>LPTSNPAQELEARQLGRTTRDDLINGNSASCADVIFIYARGSTETGNLGTLGPSIASNLESAFGKDGVWIQGVGGAYRATLGDNALPRGTSSAAIREMLGLFQQANTKCPDATLIAGGYSQGAALAAASIEDLDSAIRDKIAGTVLFGYTKNLQNRGRIPNYPADRTKVFCKTGDLVCTGSLIVAAPHLAYGPDARGPAPEFLIEKVRAVRG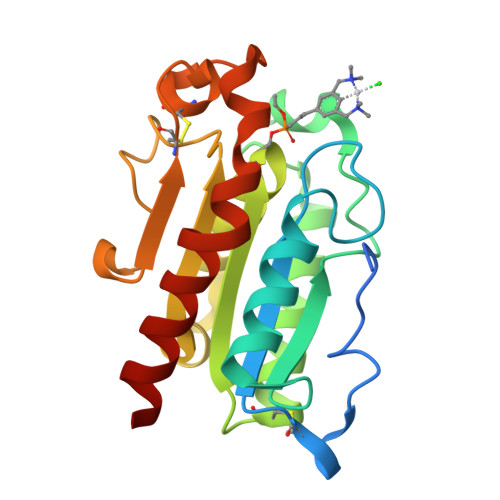SA[2x]> EPVEEEDPFFKVPVNKLAAAVSNFGYDLYRLRSSASPTGNVLLSPLSVATALSALSLGAEHRTESVIHRALYYDLITNPDIHSTYKELLASVTAPEKNLKSASRIVFERKLRVKSSFVAPLEKSYGTRPRILTGNPRVDLQEINNWVQAQMKGKIARSTREMPSALSILLLGVAYFKGQWVTKFDSRKTTLQDFHLDEDRTVRVPMMSDPKAILRYGLDSDLNCKIAQ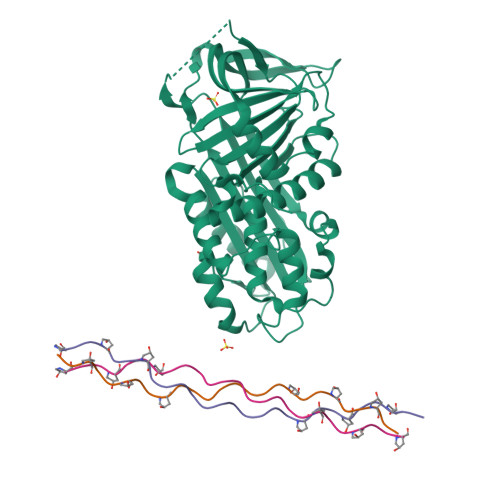LPLTGSMSIIFFLPLTVTQNLTMIEESLTSEFIHDIDRELKTIQAVLTVPKLKLSFEGELTKSLQDMKLQSLFESPDFSKITGKPVKLTQVEHRAAFEWNEEGAGSSPSGLQVRTFPLDYHLNQPFLFVLRDTDTGALLFIGRILDPSS;> YGPPGPPGPPGPPGLKGHNGLPGPPGPPGPPGPCG;> GPPGPPGPPGPKGHRGFSGLPGPPGPPGPPGCCG;> GPPGPPGPPGPKGHRGFSGLPGPPGPPGPPGCG~{N}-[2-[3,4-bis(oxidanyl)phenyl]ethyl]ethanamide 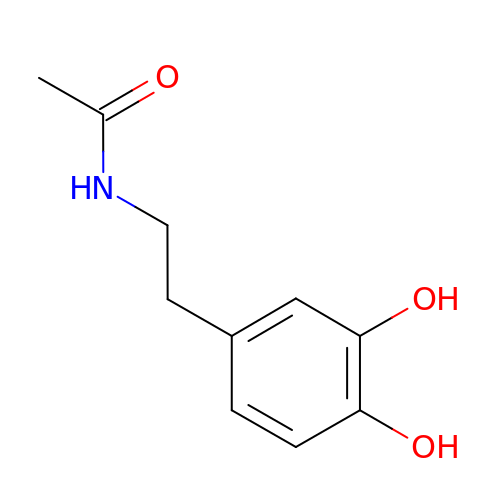| C10 H13 N O3 | OFSAJYZMIPNPHE-UHFFFAOYSA-N>[3x]SEKMVAIMKTKPGYGAELVEVDVPKPGPGEVLIKVLATSICGTDLHIYEWNEWAQSRIKPPQIMGHEVAGEVVEIGPGVEGIEVGDYVSVETHIVCGKCYACRRGQYHVCQNTKIFGVDTDGVFAEYAVVPAQNIWKNPKSIPPEYATLQEPLGNAVDTVLAGPISGKSVLITGAGPLGLLGIAVA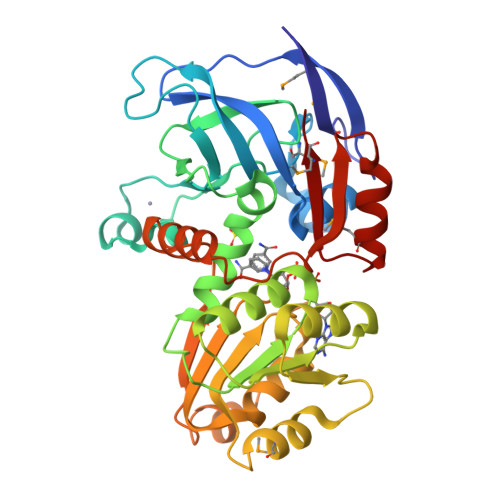KASGAYPVIVSEPSDFRRELAKKVGADYVINPFEEDVVKEVMDITDGNGVDVFLEFSGAPKALEQGLQAVTPAGRVSLLGLYPGKVTIDFNNLIIFKALTIYGITGRHLWETWYTVSRLLQSGKLNLDPIITHKYKGFDKYEEAFELMRAGKTGKVVFMLK> YRAIKGMETKREIGGYTYKVVFYENVFQDSILLGNFASQE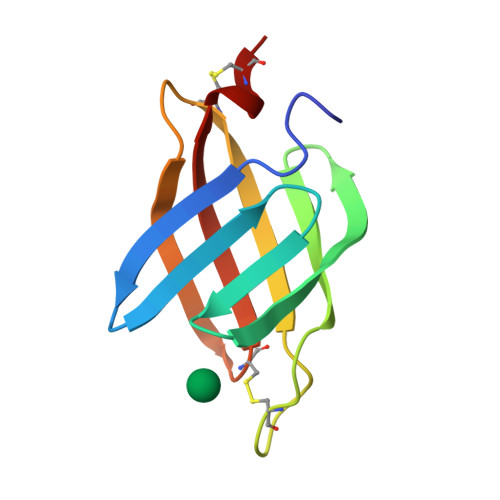GNVLKYENGQSCWNGPHRSAIVTVECGVENEIVSVLEAQKCEYLIKMKSPAACS> ATPSMMPQWSYMHISGQDASEYLSPGLVQFARATETYFSLNNKFRNPTVAPTHDVTTDRSQRLTLRFIPVDREDTAYSYKARFTLAVGDNRVLDMASTYFDIRGVLDRGPTFKPYSGTAYNALAPKGAPNPCEWDEAATALEINLEEEDDDNEDEVDEQAEQQKTHVFGQAPYSGINITKEGIQIGVEGQTPKYADKTFQPEPQIGESQWYETEINHAAGRVLKKTTPMKPCYGSYAKPTNENGGQGILVKQQNGKLESQVEMQFFSTTEATAGNGDNLTPKVVLYSEDVDIETPDTHISYMPTIKEGNSRELMGQQSMPNRPNYIAFRDNFIGLMYYNSTGNMGVLAGQASQLNAVVDLQDRNTELSYQLLLDSIGDRTRYFSMWNQAVDSYDPDVRIIENHGTEDELPNYCFPLGGVINTETLTKVKPKTGQENGWEKDATEFSDKNEIRVGNNFAMEINLNANLWRNFLYSNIALYLPDKLKYSPSNVKISDNPNTYDYMNKRVVAPGLVDCYINLGARWSLDYMDNVNPFNHHRNAGLRYRSMLLGNGRYVPFHIQVPQKFFAIKNLLLLPGSYTYEWNFRKDVNMVLQSSL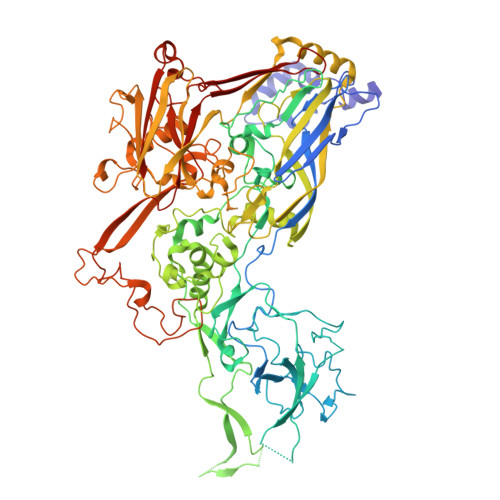GNDLRVDGASIKFDSICLYATFFPMAHNTASTLEAMLRNDTNDQSFNDYLSAANMLYPIPANATNVPISIPSRNWAAFRGWAFTRLKTKETPSLGSGYDPYYTYSGSIPYLDGTFYLNHTFKKVAITFDSSVSWPGNDRLLTPNEFEIKRSVDGEGYNVAQCNMTKDWFLVQMLANYNIGYQGFYIPESYKDRMYSFFRNFQPMSRQVVDDTKYKDYQQVGILHQHNNSGFVGYLAPTMREGQAYPANFPYPLIGKTAVDSITQKKFLCDRTLWRIPFSSNFMSMGALTDLGQNLLYANSAHALDMTFEVDPMDEPTLLYVLFEVFDVVRVHRPHRGVIETVYLRTPFSAGNATT> QFAKPEDAVKYRQSAGTLMASHFGRMTPVVKGQAPYDAAQIKANVEVLK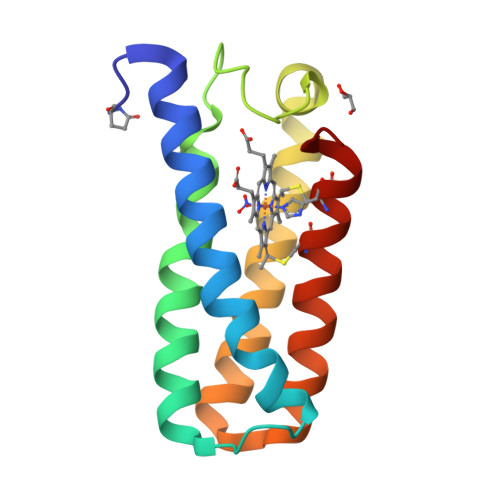TLSALPWAAFGPGTEGGDARPEIWSDAASFKQKQQAFQDNIVKLSAAADAGDLDKLRAAFGDVGASCKACHDAYRKK> MKLGVCYYPEHWPKSRWVEDAQHMRRIGIQYVRVGEFSWSTIEPTPGEL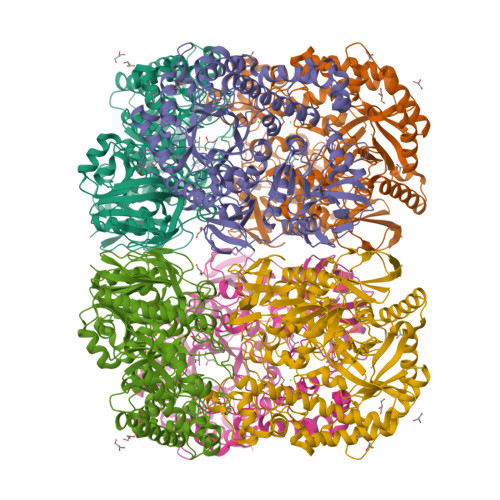HWEWLDESLDILHSQGLKVILGTPTATPPKWLVDRHPSMLAKDEAGRVRGFGSRRHYTFASLEYREECRRMVTMMAERYGHHPAVASWQTDNEYGCHDTVLSYAEADLAAFRLWLAEKYGTVEALNKAWGNVFWSMDYRSFDEIELPNLTVTEANPSHRLDFQRCCSDQVVAFNKLQVDILREHSAGRDLVHNYMGFFTAFDHHKVGQDLDVASWDSYPLGSLDKEPLYTEDEKHTYLRVGHPDAGAFHHDLYRGCGNGRLWIMEQQPGPVNWAPHNPTPADGAVRLWTWEAFSHGAELVSYFRWRQAPFGQEQMHAGLLRPDAQEAEAAKEATLVAQEVKVLAESIGLDADELMSLPSAGKVALMFDYDACWSLDIQPQSRAYRYFFWCYRMYEAMRELGLSVDIVPSNAPLDMYELLVLPAQAHITPELQNRLNSYQGVLLAGPRTGSKTETYQIPENLAPGPLASLLPLTVERVDALPEHTQPAVSGRWGAGKLKHWHEQIKTELPCLLKDDGGNPVLMGEGRHYYLGSCIDNTLLKASLAKLSEVAGLSTYYLPKGVRVRERGNVIFAFNYSSNTVVFEPQNAELVIGSMCLGAADVAIWKKQHHHHHH> MRNKIFISHATPDDNDFTRWLALKLIGLGYEVWCDILFLDKGVDFWSNIEKVI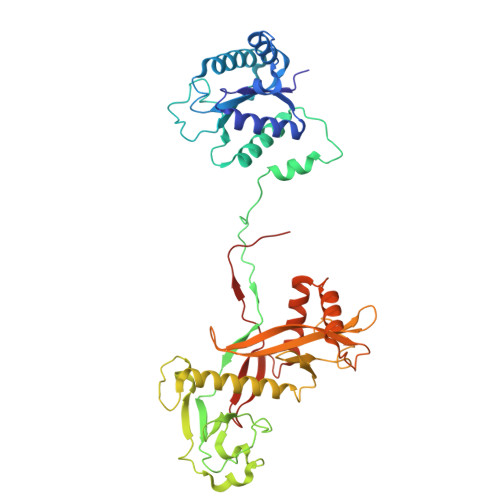REDTCKFLLVSSSYSNQREGVLKELAVAAKVKKQLKDDKFIIPLAIDEQLSYDDINIDIVRLNAIDFKMSWARGLKDILEAFEKQKVPKEVADASKSNLLYQQIFLHDKSVIEKEEIYDSNWLSILSFPEELRFHEYNWMLPKRFDVRELTFPAVRYKNYLCTFAWAYDFTYHLPKTETYHKSKTIRIPTEEILSGSYDSNFIRNAECKRLIVQLLNKAFELRMKDKEVQEYEMSNKTAYWLEKGKLEKDKFEKTMLVGKQKDKNWHFAISGASKLYPFPVLMISSHIFFTADGKKLIDSSSVQHSSRRRQGKNWWNNTWRTKLLAFIKYLSDDDTSFYLEMGSEEKVFVSNEPVKFKGNVSYNI> MPTPNIPSDFDFLDATLNLERLPVEELAELRKSEPIHWVDVPGGTGGFGDKGYWLVTKHADVKEVSRRSDVFGSSPDGAIPVYPQDMTREAVDLQRAVLLNMDAPQHTRLRKIISRGFTPRAIGRLEDELRSRAQKIAQTAAAQGAGDFVEQVSCELPLQAIAELLGVPQDDRDKLFRWSNEMTAGEDPEYADVDPAMSSFELISYAMKMAEERAVNPTEDIVTKLIEADIDGEKLSDDEFGFFVVMLAVAGNETTRNSITHGMIAFAQNPDQWELYKKERPETAADEIVRWATP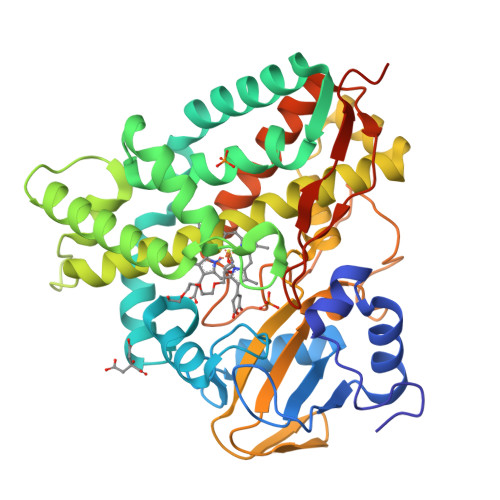VSAFQRTALEDVELGGVQIKKGQRVVMSYRSANFDEEVFEDPHTFNILRSPNPHVGFGGTGAHYCIGANLARMTINLIFNAIADNMPDLKPIGAPERLKSGWLNGIKHWQVDYTGAGKASVSGAPGTCPVA>GSHMQQWVDCEFTGRDFRDEDLSRLHTERAMFSECDFSGVNLAESQHRGSAFRNCTFERTTLWHSTFAQCSMLGSVFVACRLRPLTLDDVDFTLAVLGGNDLRGLNLT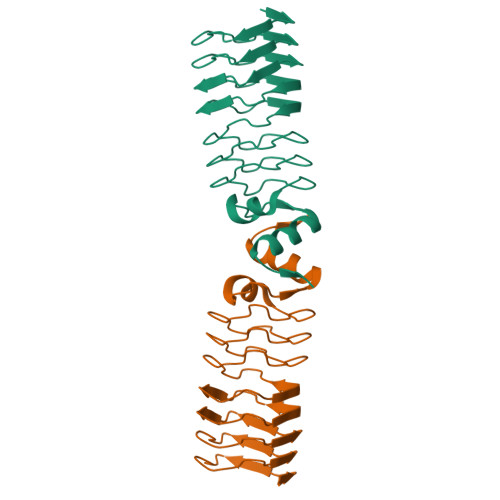GCRLRETSLVDTDLRKCVLRGADLSGARTTGARLDDADLRGATVDPVLWRTASLVGARVDVDQAVAFAAAHGLCLAGG[2x]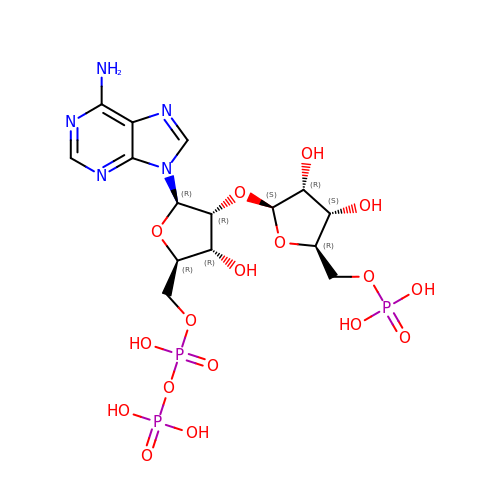[(2R,3R,4R,5R)-5-(6-aminopurin-9-yl)-4-[(2S,3R,4S,5R)-3,4-bis(oxidanyl)-5-(phosphonooxymethyl)oxolan-2-yl]oxy-3-oxidanyl-oxolan-2-yl]methyl phosphono hydrogen phosphate | C15 H24 N5 O17 P3 | GOABUQLPPRUQSR-ZQSHOCFMSA-N>UGCUCCGAGUACGA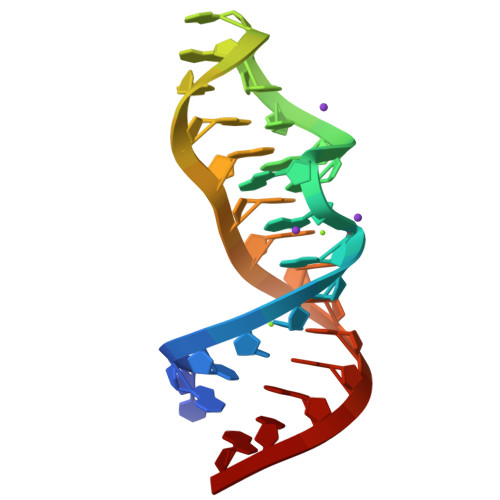GAGGAAAGGAGUG[2x]>[2x]MGSSHHHHHHSSGRENLYFQGMATITLERDGLQLVGTREEPFGEIYDMAIIFHGFTANRNTSLLREIANSLRDENIASVRFDFNGHGDSDGKFENMTVLNEIEDANAILNYVKTDPHVRNIYLVGHSQGGVVASMLAGLYPDLIKKVVLLAPAATLKGDALEGNTQGVTYNPDHIPDRLPFKDLTLGGFYLRIAQQLPIYEVSAQFTKPVCLIHGTDDTVVSPNASKKYDQIYQNST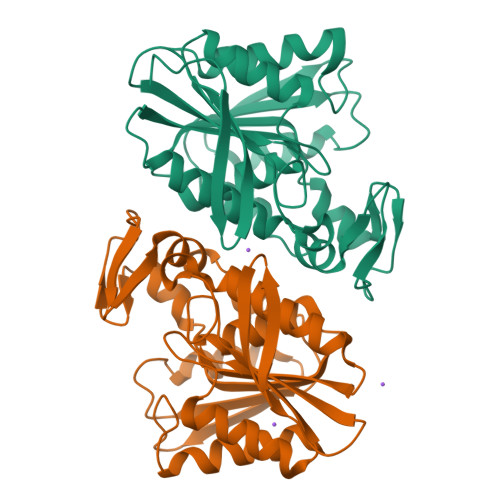LHLIEGADHCFSDSYQKNAVNLTTDFLQNNNAF> MSTALATLAGKLAERVGMDSVDPQELITTLRQTAFKGDASDAQFIALLIVANQYGLNPWTKEIYAFPDKQNGIVPVVGVDGWSRIINENQQFDGMDFEQDNESCTCRIYRKDRNHPICVTEWMDECRREP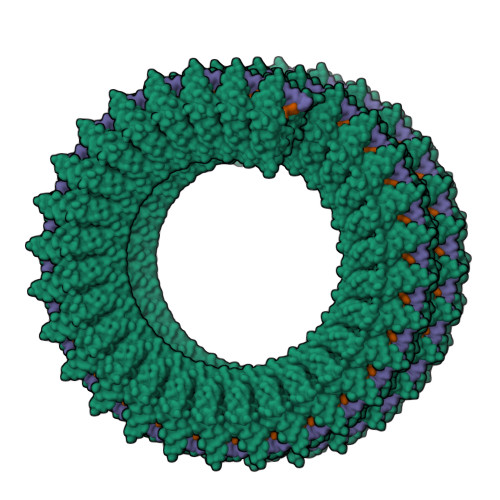FKTREGREITGPWQSHPKRMLRHKAMIQCARLAFGFAGIYDKDEAERSSHHHHHH>[2x]MPSNQEARLFLAVLVLAQVLPILVDSAAEKGFKQAFWQPLCQVSEELDDQPKGALFT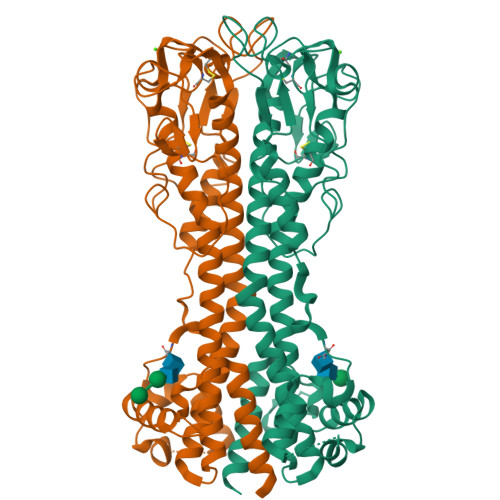LQAAASKIQKMRDAALRASIYAEINHGTNRAKAAVIVANHYAMKADSGLEALKQTLSSQEVTATATASYLKGRIDEYLNLLLQTKESGTSGCMMDTSGTNTVTKAGGTIGGVPCKLQLSPIQPKRPAATYLGKAGYVGLTRQADAANNFHDNDAECRLASGHNTNGLGKSGQLSAAVTMAAGYVTVANSQTAVTVQALDALQEASGAAHQPWIDAWKAKKALTGAETAEFRNETAGIAGKTGVTKLVEEALLKKKDSEASEIQTELKKYFSGHENEQWTAIEKLISEQPVAQNLVGDNQPTKLGELEGNAKLTTILAYYRMETAGKFEVLTQKHKPAESQQQAAETEGSCNKKDQNECKSPCKWHNDAENKKCTLDKEEAKKVADETAKDGKTGNTNTTGSSNSFVISKTPLWLAVLLF> MAHHHHHHVDDDDKDLFNKNKKLDADLLKTLDNLLKTLDNNQKQALIYFKDKLQDKKYLNDLMEQQKSFLDNLQKKKEDPDLQDRLKKTLNSEYDESQFNKLLNELGNAKAKQFLQQLHIMLQSIKDGTLTSFSSSNFNDLQNLEQKKERALQYINGKLYVEYYFYINGISNADNFFETIMEYLKT;> AGIQNDSTGKCGPPPPIDNGDITSFPLSVYAPASSVEYQCQNLYQLEGNKRITCRNGQWSEPPKCLHPCVISREIMENYNIALRWTAKQKLYSRTGESVEFVCKRGYRLSSRSHTLRTTCWDGKLEYPTCAKR

Important mechanism for complement evasion is acquisition of the main host complement inhibitor, factor H (FH). The main AP regulator in serum is Factor H (FH), which consists of 20 globular short consensus repeat domains called SCR or FH-domains. Binding of FH has also been described for RF agents, and a ligand for FH in B. hermsii was shown by Hovis et al. to be a plasmid-encoded, surface-exposed Factor H binding protein A (FhbA). By determining the 2.2 Å crystal structure of Factor H binding protein A (FhbA) from Borrelia hermsii in complex with FH domains 19–20, combined with extensive mutagenesis, we identified the structural mechanism by which B. hermsii utilizes FhbA in immune evasion.

The structure of BhFhbA (residues 44–202) reveals a compact, single-domain fold, which is composed solely of a bundle of nine α-helices. The first five α-helices (α1-α5) wrap around the core formed by α-helices 6–9 with the overall architecture of the fold resembling a curved arc or capital letter ‘L’. The structure of BhFhbA is thus a previously uncharacterized fold and further represents a novel FH-binding scaffold. The primary and biologically relevant interface in the FH20 domain has a buried surface area of 1066 Å2, as determined by the PISA server. A careful analysis of the primary interface reveals that α-helices 6–9 of BhFhbA form a hydrophobic cavity in which FH20 sits. Within the cavity, Trp1183 of FH20 surrounded by a sandwich like stack of aromatic residues sits between two BhFhbA residues: Phe154 from the hinge region and Tyr170 from helix α8. This tightly constrained binding pocket is further coordinated by the hydrophobic sidechains of α6 Met137 and Leu146 and α8 Ile171. Moreover, towards the C-terminus of FH20, Tyr199 from BhFhbA α9 forms van der Waals interactions with FH20 Val1200, with the closest approach being 3.8 Å. The structure, combined with mutagenesis and binding studies, led to the identification of a conserved aromatic residue, Phe154, that is central in binding FH. However, the interactions are different: a hydrophobic binding pocket is formed between FH20 and BhFhbA, whereas the FH20:OspE interaction is mainly electrostatic in nature and mediated by hydrogen bonds.(3R)-thiolane-3-carboxylic acid | C5 H8 O2 S | 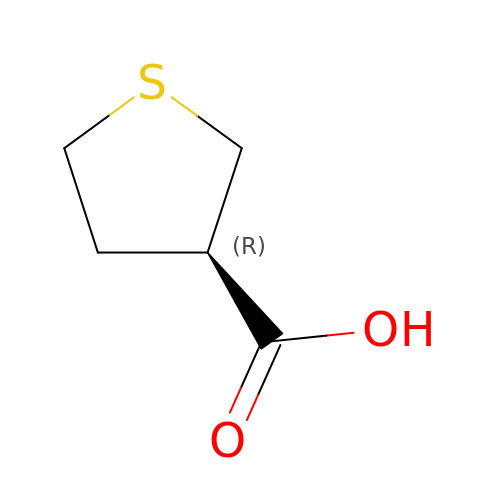BSNQHVPRAPQLSW-BYPYZUCNSA-N Fluzoparib | C22 H16 F4 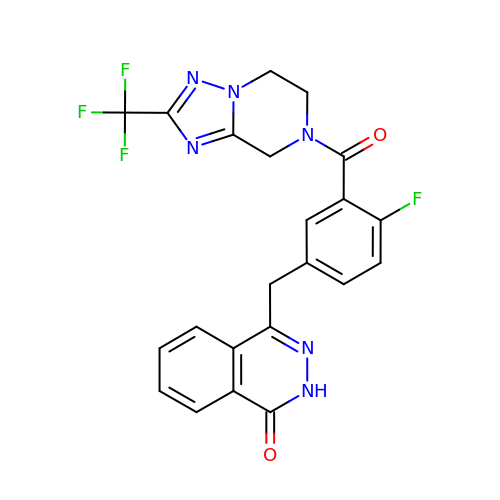N6 O2 | XJGXCBHXFWBOTN-UHFFFAOYSA-N> FQRYMEIVIVVDHSMVKKYNGDSDSIKAWVYEMINTITESY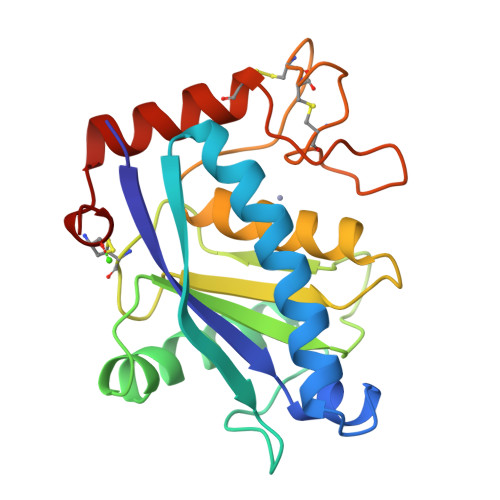SYLKIDISLSGLEIWSGKDLIDVEASAGNTLKSFGEWRAKDLIHRISHDNAQLLTATDFDGATIGLAYVASMCNPKRSVGVIQDHSSVNRLVAITLAHEMAHNLGVSHDEGSCSCGGKSCIMSPSISDETIKYFSDCSYIQCRDYIAKENPPCILN> MSETQSQTMTRPQDLSLSDINSTVEVPEGHSFWKTLLAYSGPGALVAVGYMDPGNWSTSITGGQNFQYLLLSIIVISSLLAMLLQNMAAKLGIVCQLDLAQAIRARTSRRLGFIFWILTELAIMATDIAEVIGAAIALYLLFKIPIFLAVVITVLDVFLLLLLNRIGFRKIEALVVCLIFVILFVFLYQIILSQPAWHQVAKGLIPSWASVQTSPKIGGQTPLSASLGIIGATIMPHNLFLHSAISQSRKIDRTDSSKVAEAVRFSNWDSNIQLSLAMVVNALLLIMGVAVFKSGAVQDPSFFGLYQALSNPDMVSNPVLAEAARSGVLSTLFAVALLASGQNSTITGTITGQVIMEGFIHLRLPLWLRRLVTRLIAIIPVVVCVAITSHQGSLDEHQALNNLMNNSQVFLALALPFSIVPLLMLTDSAAQMGNQFKNTRWVKVMGWLTVIILTLLNLISISSQIAGFFGDNPSSQDLLLSQVISIGIILAMIGLLIW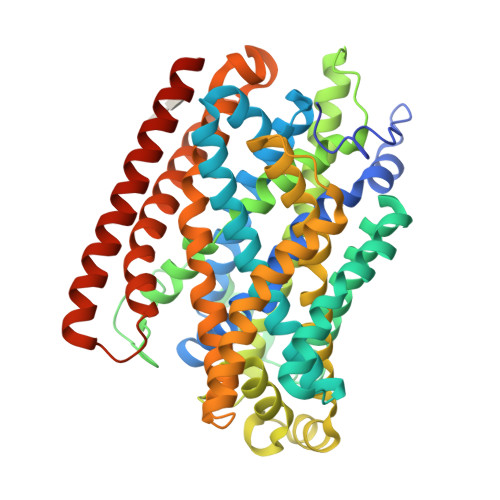TIIDIRRFTHPKQKALEVLFQ> MAASQQQASAASSAAGVSGPSSAGGPGPQQQPQPPAQLVGPAQSGLLQQQQQDFDPVQRYKMLIPQLKESLQTLMKVAAQNLIQNTNIDNGQKSSDGPIQRFDKCLEEFYALCDQLELCLRLAHECLSQSCDSAKHSP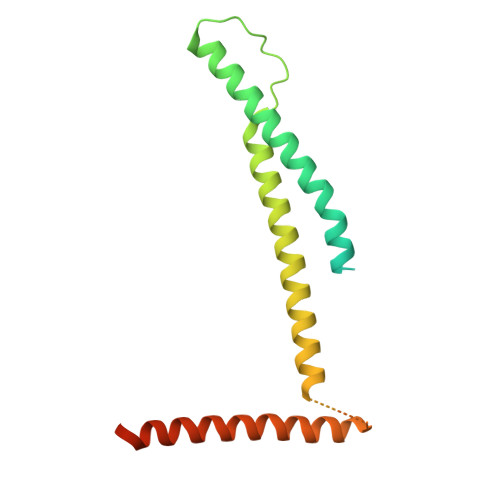TLVPTATKPDAVQPDSLPYPQYLAVIKAQISCAKDIHTALLDCANKVTGKTPAPPAGPGGTL> SRLPPATRDRLADEITFHPATAEARLLREALGRFAT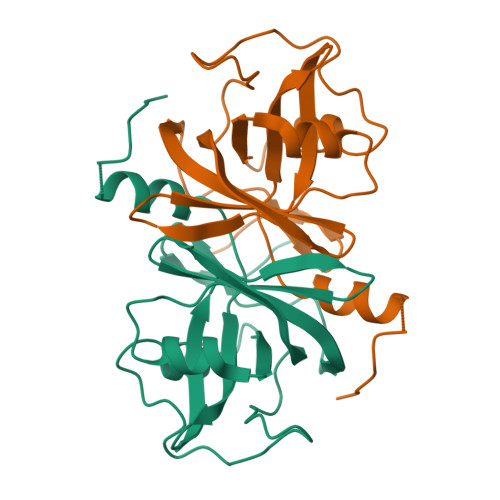GVTVVTTAGPQGPLGMTVNSFSSVSLEPPLVLWCPARTSARHAAFAEAGAWSVHVLGSEQLETCLRFTRGGRQFEGLDTVLTPEGVPVIPGVAARFDCAAHAAHEAGDHSVLIGRVLRVTVAGPGDHPLVFAAGRFGQFEPDAGLEHHHHHH The T4 bacteriophage gp41 helicase and gp61 primase assemble into a primosome to couple DNA unwinding with RNA primer synthesis for DNA replication. The domain architecture of the gp41 helicase resembles the bacterial DnaB helicase13,14 with an NTD and a RecA-like CTD that are connected by a linking helix (LH). The gp61 primase is composed of an N-terminal ZBD and a C-terminal RPD that are linked by an 18-residue flexible loop. Here we report a series of cryo-EM structures of T4 primosome assembly intermediates.

By classifying the primosome particles based on the gp61 primase regions and refining the entire primosome particles in each class, we obtained three primosome EM maps. The three primosome structures are similar, but not identical, to each other because of the asymmetry of the seam present in the gp41 helicase; they differ in the location of the two gp41 helicase dimers that bind the gp61 primase. The particle population of each pose is given in parentheses. These poses are similar, but not identical, and are referred to as binding poses 1 through 3. The poses are non-equivalent because of the asymmetric helicase structure due to the presence of a seam between subunits A and F. The gp61 ZBD and RPD bind the gp41 helicase similarly in the three binding modes with the ZBD binding to the first N-terminal helical hairpin dimer and the RPD binding to the second helical hairpin dimer in a clockwise direction when viewed from the primase side of the primosome. One gp61 primase has two binding sites on the helicase hexamer: the gp61 ZBD binds to two NTDs of one gp41 dimer, and the gp61 RPD binds to two NTDs of a second gp41 dimer. In each binding pose, the ssDNA 5′-end emerging from the gp41 helicase consistently passes between the gp61 ZBD and RPD domains. The three gp61 primase binding poses are observed in the T4 primosome in the presence of ssDNA and ATPγS. In our initial primosome structure, there was no density for the RNA primer, but the density for the ssDNA was present stretching from the gp61 ZBD to the N-terminal lobe (NTL) of the gp61 RPD; therefore, this structure may represent an ssDNA-scanning configuration of the primosome in search of a priming recognition sequence. The first state is observed in the WT primosome in which the primase interacts with the ssDNA template in three largely equivalent poses.

>[6x]MVEIILSHLIFDQAYFSKVWPYMDSEYFESGPAKNTFKLIKSHVNEYHSVPSINALNVALENSSFTETEYSGVKTLISKLADSPEDHSWLVKETEKYVQQRAMFNATSKIIEIQTNAELPPEKRNKKMPDVGAIPDIMRQALSISFDSYVGHDWMDDYEARWLSYMNKARKVPFKLRILNKITKGGAETGTLNVLMAGVNVGKSLGLCSLAADYLQLGHNVLYISMEMAEEVCAKRIDANMLDVSLDDIDDGHISYAEYKGKMEKWREKSTLGRLIVKQYPTGGADANTFRSLLNELKLKKNFVPTIIIVDYLGICKSCRIRVYSENSYTTVKAIAEELRALAVETETVLWTAAQVGKQAWDSSDVNMSDIAESAGLPATADFMLAVIETEELAAAEQQLIKQIKSRYGDKNKWNKFLMGVQKGNQKWVEIEQDSTPTEVNEVAGSQQIQAEQNRYQRNESTRAQLDALANELKF;> MSSIPWIDNEFAYRALAHLPKFTQVNNSSTFKLRFRCPVCGDSKTDQNKARGWYYGDNNEGNIHCYNCNYHAPIGIYLKEFEPDLYREYIFEIRKEKGKSRPIEKPKELPKQPEKKIIKSLPSCVRLDKLAEDHPIIKYVKARCIPKDKWKYLWFTTEWPKLVNSIAPGTYKKEISEPRLVIPIYNANGKAESFQGRALKKDAPQKYITIEAYPEATKIYGVERVKDGDVYVLEGPIDSLFIENGIAITGGQLDLEVVPFKDRRVWVLDNEPRHPDTIKRMTKLVDAGERVMFWDKSPWKSKDVNDMIRKEGATPEQIMEYMKNNIAQGLMAKMRLSKYAKI> TGMSREEVESLIQEVLEVYPEKARKDRNKHLAVNDPAVTQSKKCIISNKKSQPGLMTIRGCAYAGSKGVVWGPIKDMIHISHGPVGCGQYSRAGRRNYYIGTTGVNAFVTMNFTSDFQEKDIVFGGDKKLAKLIDEVETLFPLNKGISVQSECPIGLIGDDIESVSKVKGAELSKTIVPVRCEGFRGVSQSLGHHIANDAVRDWVLGKRDEDTTFASTPYDVAIIGDYNIGGDAWSSRILLEEM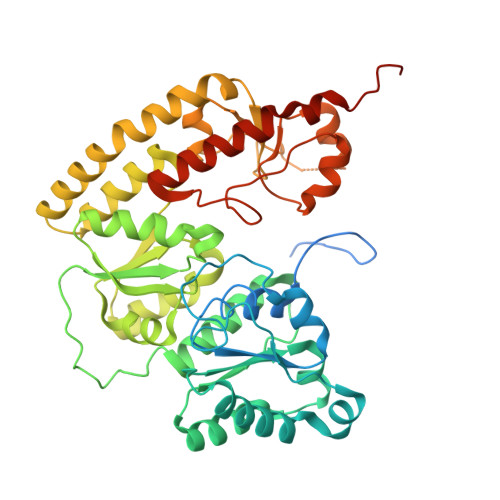GLRCVAQWSGDGSISEIELTPKVKLNLVHCYRSMNYISRHMEEKYGIPWMEYNFFGPTKTIESLRAIAAKFDESIQKKCEEVIAKYKPEWEAVVAKYRPRLEGKRVMLYIGGLRPRHVIGAYEDLGMEVVGTGYEFAHNDDYDRTMKEMGDSTLLYDDVTGYEFEEFVKRIKPDLIGSGIKEKFIFQKMGIPFREMHSWDYSGPYHGFDGFAIFARDMDMTLNNPCWKKLQAPWEASEGAEKVAASA8-[3-chloranyl-5-[1-methyl-2,2-bis(oxidanylidene)-3~{H}-2,1-benzothiazol-5-yl]pyridin-4-yl]-1-oxa-3,8-diazaspiro[4.5]decan-2-one 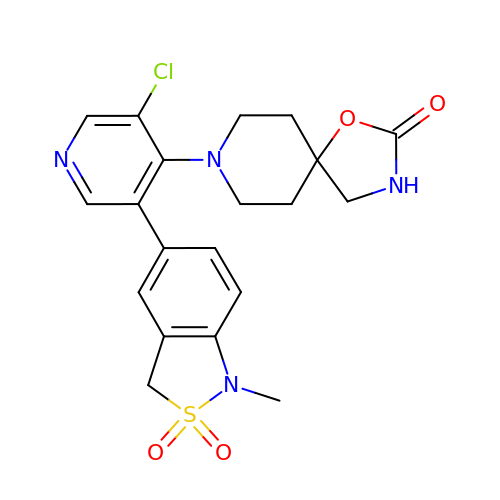| C20 H21 Cl N4 O4 S | ZNMSRFYDOSAZLZ-UHFFFAOYSA-N> MASWSHPQFEKSGGGGGENLYFQGAVLALERHFEKVEEILKKYGYKRENLIKILLEIQEIYRYLPEDVINYVSTAMGIPPAKIYGVATFYAQFSLKPKGKYTIMVCDGTACHMAGSPEVLKAI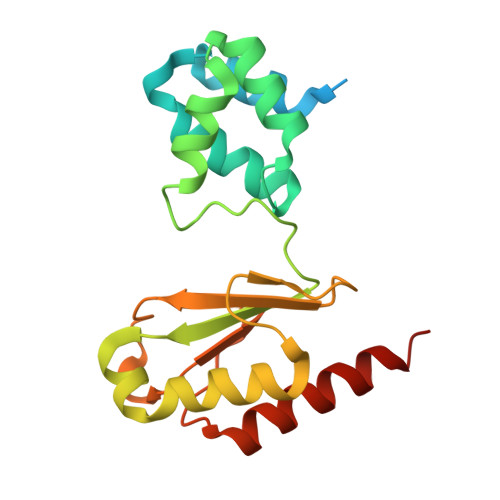EEETGLTPGNVTEDLMFSLDQVGCLGACALAPVMVINGEVYGNLTADKVKEILRKIKEKERESANV> MRPIRMYKNNQERTNLKHQEINEEQQNEQTTSNQGFTRSDNSGKINIERISSSRNQITDGKTVSSYSKIETNRSSQDSVQHGGSSITYTSDTTGNPRITNARTNNDETHATGPIEDLNSTSHGREPEIESFADRAELAMMIQGMTVGALTVQPMRSIRSTFANLANVLIFHDVFTTEDKPSAFIEYHSDEMIVNMPKQTYNPIDNLAKILYLPSLEKFKYGTGIVQLNYSPHISKLY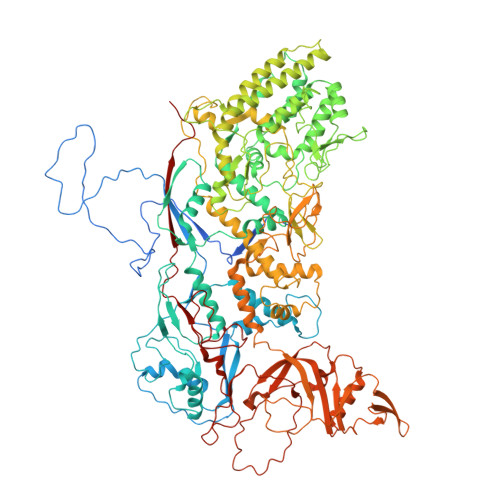QNTNNIINTITDGITYANRTEFFIRVMVLMMMDRKILTMEFYDVDTSAISNTAILPTIPTTTGVSPLLRIDTRTEPIWYNDAIKTLITNLTIQYGKIKTVLDANAVKRYSVVGYPIDQYRAYLYNHNLLEYLGKKVKREDIMSLIKALSYEFDLITISDLEYQNIPKWFSDNDLSRFIFSICMFPDIVRQFHALNIDYFSQANVFTVKSENAIVKMLNSNQNMEPTIINWFLFRICAIDKTVIDDYFSLEMTPIIMRPKLYDFDMKRGEPVSLLYILELILFSIMFPNVTQHMLGQIQARILYISMYAFRQEYLKFITKFGFYYKIVNGRKEYIQVTNQNERMTENNDVLTGNLYPSLFTDDPTLSAIAPTLAKIARLMKPTTSLTPDDRAIAAKFPRFKDSAHLNPYSSLNIGGRTQHSVTYTRMYDAIEEMFNLILRAFASSFAQRPRAGVTQLKSLLTQLADPLCLALDGHVYHLYNVMANMMQNFIPNTDGQFHSFRACSYAVKDGGNIYRVVQNGDELNESLLIDTAIVWGLLGNTDSSYGNAIGATGTANVPTKVQPVIPTPDNFITPTIHLKTSIDAICSVEGILLLILSRQTTIPGYEDELNKLRTGISQPKVTERQYRRARESIKNMLGSGDYNVAPLHFLLHTEHRSTKLSKPLIRRVLDNVVQPYVANLDPAEFENTPQLIENSNMTRLQIALKMLTGDMDDIVKGLILHKRACAKFDVYETLTIPTDVKTIVLTMQHISTQTQNNMVYYVFLIDGVKILAEDIKNVNFQIDITGIWPEYVITLLLRAINNGFNTYVSMPNILYKPTITADVRQFMNTTKAETLLISNKSIVHEIMFFDNALQPKMSSDTLALSEAVYRTIWNSSIITQRISARGLMNLEDARPPEAKISHQSELDMGKIDETSGEPIYTSGLQKMQSSKVSMANVVLSAGSDVIRQAAIKYNVVRTQEIILFE> RSRIFKIIVIGDSNVGKTCLTYRFCAGRFPDRTEATIGVDFRERAVDIDGERIKIQLW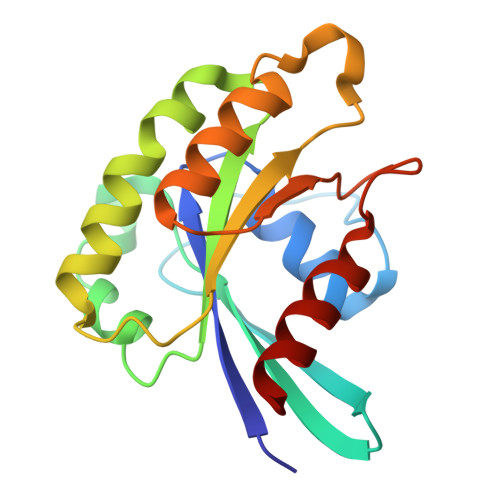DTAGLERFRKSMVQHYYRNVHAVVFVYDMTNMASFHSLPAWIEECKQHLLANDIPRILVGNKCDLRSAIQVPTDLAQKFADTHSMPLFETSAKNPNDNDHVEAIFMTLAHKLKSH METHYLPENTA(OXYETHYL) HEPTADECANOATE 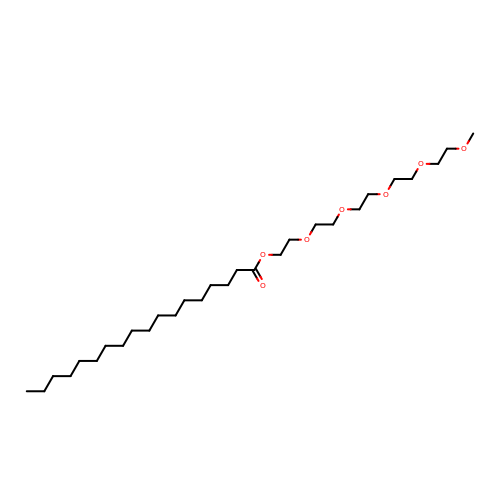| C29 H58 O7 | AKUODCGCIHXMIY-UHFFFAOYSA-N>AEAGITGTWYNQLGSTFIVTAGADGALTGTYESAVGNAESRYVLTGRYDSAPATDGSGTALGWTVAWKNNYRNDH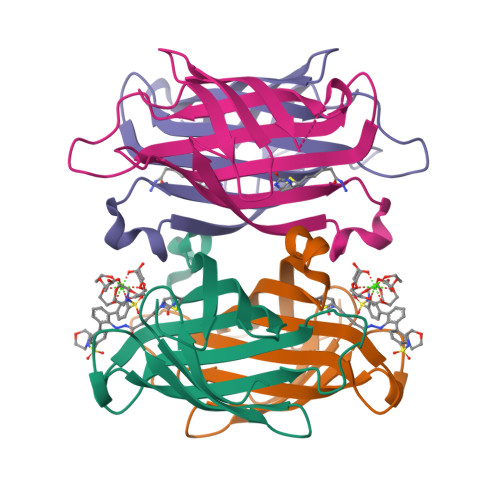SATTWSGQYVGGAEARINTQWLLTSGTTEANAWKSTLVGHDTFTKVKPSAAS[4x]> GSHMKKVIIAGNGPSLKEIDYSRLPNDFDVFRCNQFYFEDKYYLGKKCKAVF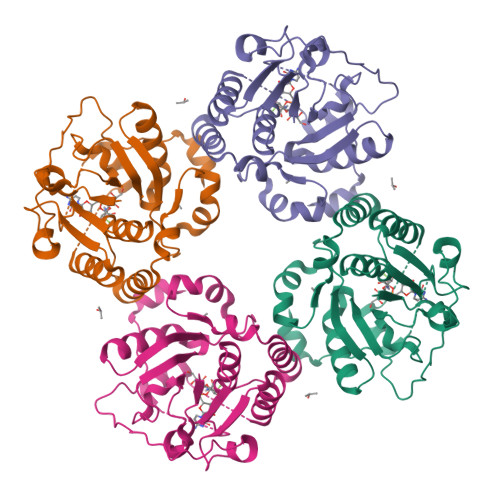YNPSLFFEQYYTLKHLIQNQEYETELIMCSNYNQAHLENENYVKTFYDYFPDAHLGYDFFKQLKDFNAYFKFHEIYFNQRITSGVYMCAVAIALGYKEIYLSGIDFYQNGSSYAFDTKQKNLLKLAPNFKNDNSHYIGHSKNTDIKALEFLEKTYKIKLYCLCPNSLLANFIGLAPNLNSNFIIQEKNNYTKDILIPSSEAYGKFSKNIN> MASRADKASSIELKFD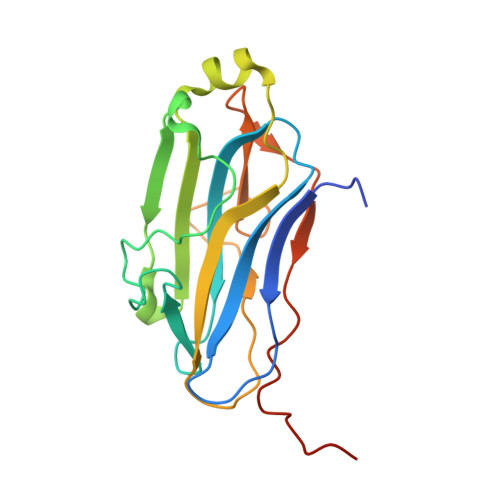RNKGEVGDILIGTVRINNIKNFAGFQVNIVYDPKVLMAVDPETGKEFTSSTFPPGRTVLKNNAYGPIQIADNDPEKGILNFALAYSYIAGYKETGVTEESGIIAKIGFKILQKKSTAVKFQDTLSMPGAILGTQLFDWDGEVITGYEVIQPDVLSLGDEPYEVEHHHHHH>SMQRTVARDITLLECVGKGRYGEVWRGSWQGENVAVKIFSSRDEKSWFRETELYNTVMLRHENILGFIASDMTSRHSSTQLWLITHYHEMGSLYDYLQLTTLDTVSCLRIVLSIASGLAHLHIEIFGTQGKPAIAHRDLKSKNILVKKNGQCCIADLGLAVMHSQSTNQLDVGNNPRVGTKRYMAPEVLDETIQVDCFDSYKRVDIWAFGLVLWEVARRMVSNGIVEDYKPPFYDVVPNDPSFEDMRKVVCVDQQRPNIPNRWFSDPTLTSLAKLMKECW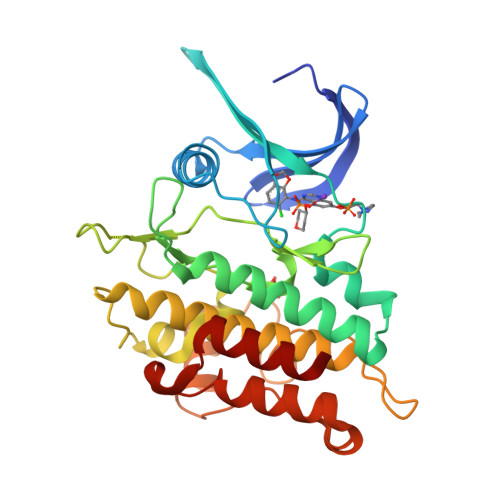YQNPSARLTALRIKKTLTKID[4x]> MTSYTYQATPMDGTLKTMLERWAADSNMQLSYNLPSDYTLIGPVSAISTTSVQQAATELSAVYAAQGVSVSVSANKLLVQPVPVS

In well-characterized T4SSs, VirB7 is a lipoprotein attached to the periplasmic side of the outer membrane. In order to understand the unique structural features of Xanthomonad VirB7, we have solved the solution nuclear magnetic resonance (NMR) and X-ray crystal structures of XAC2622, which we now call VirB7XAC2622, and studied its interaction with VirB9. VirB7XAC2622 presents all of the characteristics of VirB7: predicted signal peptide and lipobox sequences followed by a short and extended region that contains the VirB9 binding site. However, unlike other VirB7 proteins, VirB7XAC2622 has an extra domain whose topology is strikingly similar to that of N0 domains found in proteins from different multi-subunit complexes involved in transport across the bacterial outer membrane.

To better characterize the globular domain, we cloned and purified a recombinant fragment encompassing residues 51–134 (VirB7XAC2622_51–134) which was submitted to crystallization trials that resulted in large plates which belong to space group C2221 and diffracted up to 1.0 Å. Molecular replacement was performed using the solution structure of the VirB7XAC2622 globular domain as the search model. There was clear electron density for all residues, with the exception of the first amino acid (threonine 51) and residues 122 and 123 in the loop between β4 and β5. As expected, the crystal structure is very similar to the NMR ensemble, displaying an average root mean square deviation (RMSD) for the backbone heavy atoms and all heavy atoms of 1.05±0.05 Å and 1.61±0.06 Å for residues 53–130, and excellent agreement with the backbone 1H-15N RDCs [Q factor of 0.187 (regular secondary structures only) and 0.272 (all residues)]. The globular domain is composed of two α-helices sandwiched between a mixed three stranded β-sheet on one side and an antiparallel two-stranded β-sheet plus a short 310 helix on the other. The VirB7XAC2622 globular domain has no significant sequence similarity to proteins of known structure. In addition to the canonical VirB7-like N-terminal region, VirB7XAC2622 has a C-terminal region that includes a globular domain (residues 52–133). This globular domain does not interact with VirB9XAC2620_154–255 but does interact with an extended region (residues 42–49) that immediately precedes the globular domain in another VirB7XAC2622 molecule, leading to the formation of homo-oligomers. As expected, no cross-links were observed when the experiment was performed using VirB7XAC2622_51–134 which lacks the disordered N-terminal region.4-({4-[(2-bromophenyl)amino]pyrimidin-2-yl}amino)benzoic 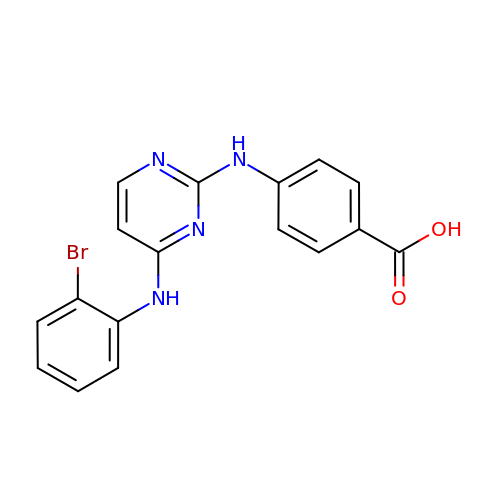acid | C17 H13 Br N4 O2 | NCXZWZMYZVWHNN-UHFFFAOYSA-N> MSELEKAVVALIDVFHQYSGREGDKHKLKKSELKELINNELSHFLEEIKEQEVVDKVMETLDSNGDGECDFQEFMAFVAMITTACHEFFEHE;> TKIDWNK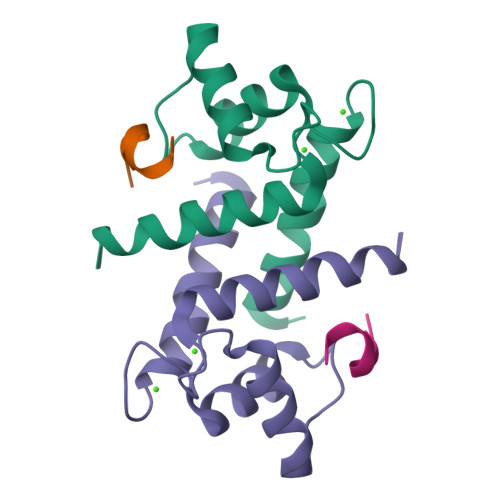IL> GMATPKKDVYTIASDNSFAPFEFQNDDKQFTGIDVDLLNAIAKNQGFKLKWNFIGFQAAVDSVQSGHADGMMSGMSITDARKQVFDYGSPYYSSNLTIATSSTDDSIKSWKDLKGKTLGAKNGTASFDYLNAHAKEYGYTVKTFTDATTMYSSLNNGSINALMDDEPVIKYAIKQGQKFATPIKPIPDGQYGFAVKKGSNPELIEMFNNGLANLRANGEYDKIIDKYLES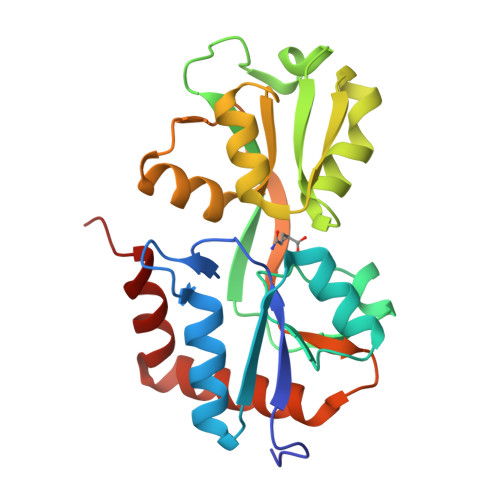DA>[2x]MVNAEEQQYLNLVQYIINHGEDRPDRTGTGTLSVFAPSPLKFSLRNKTFPLLTTKRVFIRGVIEELLWFI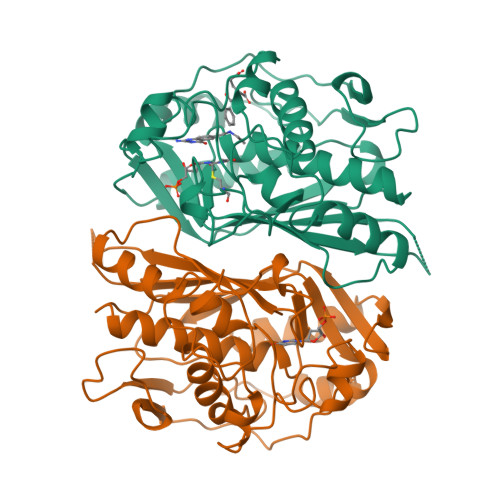RGETDSLKLREKNIHIWDANGSREYLDSIGLTKRQEGDLGPIYGFQWRHFGAEYIDCKTNYIGQGVDQLANIIQKIRTSPYDRRLILSAWNPADLEKMALPPCHMFCQFYVHIPSNNHRPELSCQLYQRSCDMGLGVPFNIASYALLTCMIAHVCDLDPGDFIHVMGDCHIYKDHIEALQQQLTRSPRPFPTLSLNRSITDIEDFTLDDFNIQNYHPYETIKMKMSI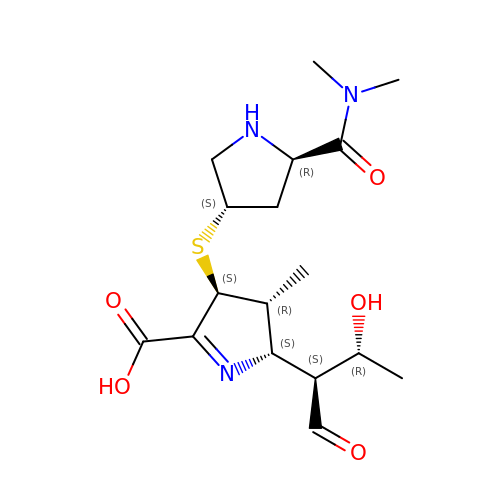(2S,3R,4S)-4-{[(3S,5R)-5-(dimethylcarbamoyl)pyrrolidin-3-yl]sulfanyl}-2-[(2S,3R)-3-hydroxy-1-oxobutan-2-yl]-3-methyl-3,4-dihydro-2H-pyrrole-5-carboxylic acid | C17 H27 N3 O5 S | UUIYVKJXUXGPKB-DKLFCYGSSA-N>[2x]MSLYRRLVLLSCLSWPLAGFSATALTNLVAEPFAKLEQDFGGSIGVYAMDTGSGATVSYRAEERFPLCSSFKGFLAAAVLARSQQQAGLLDTPIRYGKNALVPWSPISEKYLTTGMTVAELS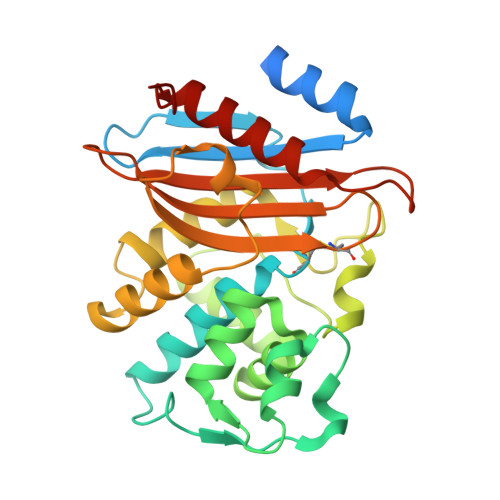AAAVQYSDNAAANLLLKELGGPAGLTAFMRSIGDTTFRLDRWELELNSAIPGDARDTSSPRAVTESLQKLTLGSALAAPQRQQFVDWLKGNTTGNHRIRAAVPADWAVGDKTGTCGVYGTANDYAVVWPTGRAPIVLAVYTRAPNKDDKHSEAVIAAAARLALEGLGVNGQQ Despite the ‘rule of thumb’ that blood feeders from independent evolutionary lineages utilize different protein families for various salivary functions, the saliva of sand flies contains apparent homologs of the two-domain long-form D7 proteins of mosquitoes. In this study we demonstrate, using binding studies and bioassays, that the sand fly long-form D7s do in fact bind both cysteinyl leukotrienes and thromboxanes, and thereby serve as anti-inflammatory and anti-hemostatic agents in both sandflies and mosquitoes. In this study we show that the long-form D7 proteins from sand flies are functionally like their counterparts in mosquito saliva and share a conserved structure. Consistent with these structural observations, the sand fly proteins were found to perform the same anti-inflammatory and anti-platelet functions as their mosquito counterparts through the binding of cysteinyl leukotrienes and TXA2 in the N-terminal domain, but do not bind biogenic amines, as this function is performed by the yellow proteins.

The structure of ABI15936 was determined using single anomalous diffraction methods with a selenomethionine-substituted variant protein prepared in E. coli. An initial model containing two protein monomers was built using the experimental electron density map and then positioned into a wild-type data set by molecular replacement. As suggested by sequence comparisons, the protein is made up of two linked odorant binding protein (OBP) domains with a well-ordered domain interface fixing their relative orientations. The N-terminal domain contains a hydrophobic channel leading from the surface to the interior of the protein that is much like the eicosanoid binding pocket in Aedes and Anopheles long-form D7 proteins. The C-terminal domain appears generally like those of the mosquito proteins but does not contain the biogenic amine binding pocket seen in AeD7, the Ae. aegypti long D7 protein that binds both eicosanoids and biogenic amines. The N-terminal domain of ABI15936 contains two disulfide bonds that are conserved in the mosquito proteins. These link Cys 17 with Cys 47 and Cys 45 with Cys 93. The C-terminal domain contains three disulfides linking Cys 143 with Cys 159, Cys 155 with Cys 202 and Cys 192 with Cys 211. Although ABI15936 was crystallized in the absence of any potential natural ligands, electron density was observed indicative of a non-protein molecule occupying the N-terminal domain binding site. This was determined after refinement of the protein complex to be the detergent Triton X-100, which was retained through the steps of protein purification.

>[2x]MWRYPRNADQTFWAFRTCQRQSEGAKSLREWYRWNLPNDEDTHCYVKCVWLHLGLYNEQNKSLRVDRIMEQFNSRSVAIPGGINTISGPTDGTCKDIYDKTINFFNNNVNDLRTAFYGIKKLSDEWFTQNSNTKPKGTKISDFCNAENREKGGADCQHACSAYYYRLVDEDNEPIHFRNLNILGITDEQFASCVKASKNKQGCKVADTMYNCVEKHNSQALKILDNQSPTY> GAMAKTLDKKRIEQIKSECLRIYRIGIGHPSNSEILKYATEEEKKILIPILRKKPVRTISGVAVVAVMTSPAKCPHGKCIFCPGGLDSVFGDVPQSYTGREPATMRGLMFNFDPYLQTRARIEQLEKVGHPTDKIELIIMGGTFPAREIEYQDWFIKRCLDAMNERESKSLEEAQKINETAKHRCVALCIETRPDYCSEKEINQMLKLGATRVELGVQSIYNEILKLCKRGHSVEDTIKATQLLKDSGLKVSYHLMPGMPGSSIEMDKKMFKEIFTNPDFMPDMVKIYPCLVIEGTELYEMWKRGEFKPYREEEAIEVISYAKSIMPKWVRTSRIQRDIPATVIVDGVKKSNLGELVYKYMEKKGLRCRCIRCREVGHVYYKKGILPDPEHIKLVREDYEASGGTEIFLSFEDVKNDILIAFLRLRDPYKPFRKEIDDKTMLVRQLHVFGWEKALTRDIKEVSWQHMGYGRMLMKEAERIAKEEFGKKKILVTSGIGVREYYRKLGYKRVGAYMGKEL

Elp3 acts as the catalytic subunit, but the loss of any of the six subunits results in hypo-modified U34 tRNAs in yeast, indicating that the complete integrity of the complex is important for its function. The enzymatically active Elp3 subunit of Elongator contains two functional domains, utilizes multiple cofactors, and conducts a unique uridine base modification specifically found only at the wobble base position of tRNAs. The two domains form a cleft that contains several highly conserved basic residues, which bind and accommodate the tRNA anticodon stem loop (ASL). The current model of a radical based Elp3-mediated cm5-modification reaction is proposed as follows (i) Elp3 recruits SAM and cleaves it to generate a 5’deoxyadenosine radical (5’-dA) in the rSAM domain, (ii) Elp3 hydrolyzes acetyl-CoA in the KAT domain and (iii) an acetyl radical is formed by the products of the two domains and (iv) is transferred onto the C5 position of U34 in the bound tRNA molecule.

Although DmcElp3 and Methanocaldococcus infernus Elp3 (MinElp3) share 50% sequence identity, MinElp3 harbors an extended N-terminus (aa 1–75). We further generated five different N-terminally truncated versions (MinElp3Δ1–19, MinElp3Δ1–41, MinElp3Δ1–46, MinElp3Δ1–54, MinElp3Δ1–68) to facilitate crystallization. We used full length and truncated versions of purified MinElp3 in crystallization trials and obtained well-diffracting crystals for monomeric MinElp3Δ1–19, MinElp3Δ1–46, and MinElp3Δ1–54. We solved their structures using a poly-alanine model of DmcElp3 via molecular replacement at 1.9 Å, 1.9 Å, and 2.1 Å resolution, respectively. Although all three versions contained various lengths of the N-terminus and also showed no signs of degradation, we could observe interpretable electron density only starting from residue V72 in all collected and refined datasets. Therefore, we believe that the N-terminus adopts a highly flexible conformation in the absence of substrate tRNAs. The overall structure and domain arrangement and interface between the rSAM and KAT domains of MinElp3 are almost identical to DmcElp3. The main difference relates to the Fe–S cluster loop region (aa 87–123) and the Fe–S cluster itself, which were both completely unstructured in all monomeric MinElp3s. In our MinElp3 structures, we could not locate any bound Zn-ions and instead observed the formation of a disulfide bond between C384 and C389. In addition, we observed that the acetyl-CoA blocking loop (aa 466–486) is positioned outside of the acetyl-CoA binding pocket, interacting with the last visible residues of the N-terminus and also contacting a neighboring symmetry mate.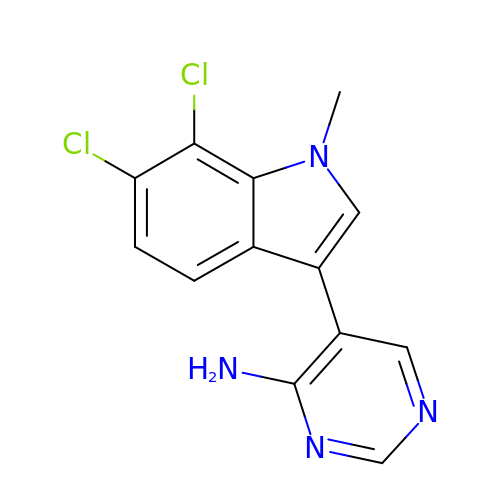5-[6,7-bis(chloranyl)-1-methyl-indol-3-yl]pyrimidin-4-amine | C13 H10 Cl2 N4 | QPVJIMUMKNWEER-UHFFFAOYSA-N>RNLLTNGEGLYAGQSLDVEPYHFIMQEDCNLVLYDHSTSVWASNTGILGKKGCKAVLQSDGNFVVYDAEGRSLWASHSVRGNGNYVLVLQEDGNVVIYGSDIWSTGTYK[2x];>[2x]RNILMNDEGLYAGQSLDVEPYHLIMQEDCNLVLYDHSTAVWT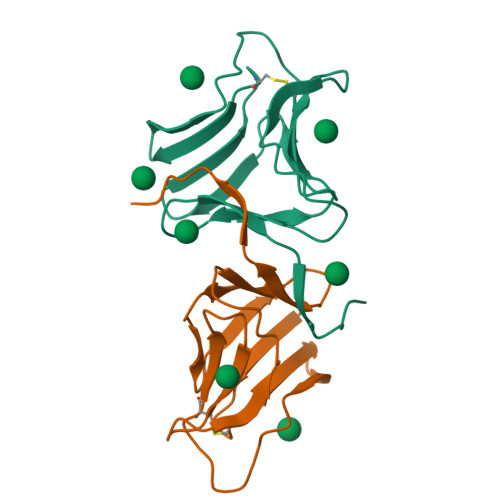TNTDIPGKKGCKAVLQSDGNFVVYDAEGRSLWASHSVRGNGNYVLVLQEDGNVVIYGSDIWSTNTYK(3~{R},5~{R},7~{a}~{S})-2,2-dimethyl-5-(sulfanylmethyl)-3,5,7,7~{a}-tetrahydro-[1,3]thiazolo[4,3-b][1,3]thiazole-3-carboxylic 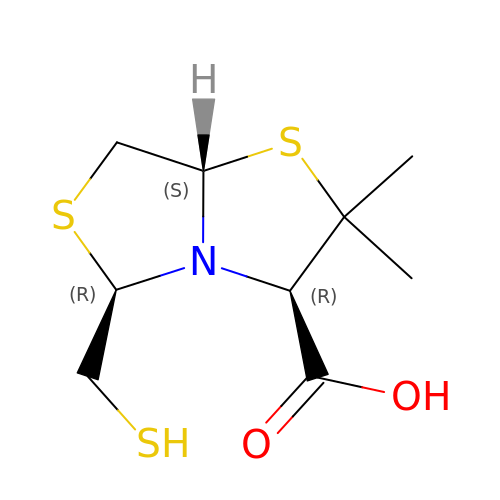acid | C9 H15 N O2 S3 | IKSIYRPSHTUWIX-DSYKOEDSSA-N The cytochrome c maturation system I, consisting of eight membrane proteins (CcmABCDEFGH), results in the attachment of heme to cysteine residues of cytochrome c proteins. CcmABCD represents an ABC transporter complex using the energy of ATP hydrolysis for the transfer of heme from one binding partner (CcmC) to another (CcmE). Our cryo-EM structures reveal that CcmA2B2 form a homodimer which is an ABC transporter analog. CcmC which harbors the heme-binding site is attached to two CcmBs with two coupling helices TM4 and TM5 on CcmC, respectively.

Three-dimensional classification in cryo-EM studies reveals two major states of apoCcmABCD and CcmABCD in complex with ATP and heme, and one state of CcmABCD complexed with AMP-PNP. In one of the apoCcmABCD conformations, each CcmA binds one inorganic phosphate and the two CcmABs tightly contact to form a “full-closed” conformation. In the closed-NBD state of apoCcmABCD bound with inorganic phosphates, N36A is H-bonded with the phosphate, and A156A, G130A in the other CcmA (right zoomed in panel). For WT CcmABCD, the protein changes to open-NBD state to break these H-bonds and release the phosphate for the next cycle. Superposition of each of the closed NBD states of CcmABCD indicate nearly identical structures (e.g., with two ATPs or two inorganic phosphates or two AMP-PNPs). Our structures also reveal substantial conformational changes upon binding of ATP (to CcmA) and heme (to CcmC): closed NBD conformation when bound with two inorganic phosphates, two ATPs or two AMP-PNPs; open NBD conformation when it is ligand-free; and semi-open NBD when bound with one ATP.

>MGMLEARELLCERDERTLFSGLSFTLNAGEWVQITGSNGAGKTTLLRLLTGLSRPDAGEVLWQGQPLHQVRDSYHQNLLWIGHQPGIKTRLTALENLHFYHRDGDTAQCLEALAQAGLAGFEDIPVNQLSAGQQRRVALARLWLTRATLWILDEPFTAIDVNGVDRLTQRMAQHTEQGGIVILTTHQPLNVAESKIRRISLTQTRAA[2x];>MMFWRIFRLELRVAFRHSAEIANPLWFFLIVITLFPLSIGPEPQLLARIAPGIIWVAALLSSLLALERLFRDDLQDGSLEQLMLLPLPLPAVVLAKVMAHWMVTGLPLLILSPLVAMLLGMDVYGWQVMALTLLLGTPTLGFLGAPGVALTVGLKRGGVLLSILVLPLTIPLLIFATAAMDAASMHLPVDGYLAILGALLAGTATLSPFATAAALRISIQ[2x];> MWKTLHQLAIPPRLYQICGWFIPWLAIASVVVLTVGWIWGFGFAPADYQQGNSYRIIYLHVPAAIWSMGIYASMAVAAFIGLVWQMKMANLAVAAMAPIGAVFTFIALVTGSAWGKPMWGTWWVWDARLTSELVLLFLYVGVIALWHAFDDRRLAGRAAGILVLIGVVNLPIIHYSVEWWNTLHQGSTRMQQSIDPAMRSPLRWSIFGFLLLSATLTLMRMRNLILLMEKRRPWVSELILKRGRK;> MTPAFASWNEFFAMGGYAFFVWLAVVMTVIPLVVLVVHSVMQHRAILRGVAQQRAREARLRAAQQQEAA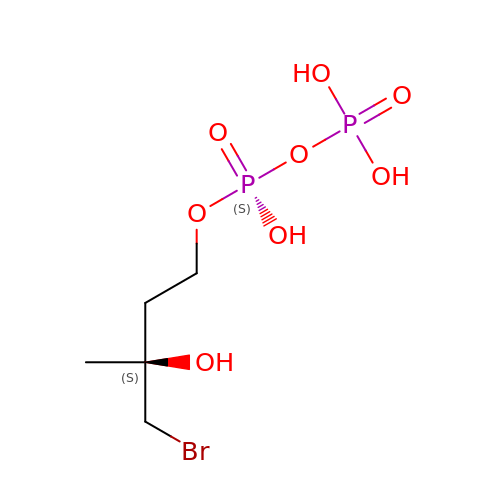(S)-4-BROMO-3-HYDROXY-3-METHYLBUTYL DIPHOSPHATE | C5 H13 Br O8 P2 | YKAYCWPQDPILSA-YFKPBYRVSA-N1H-indazol-7-amine | C7 H7 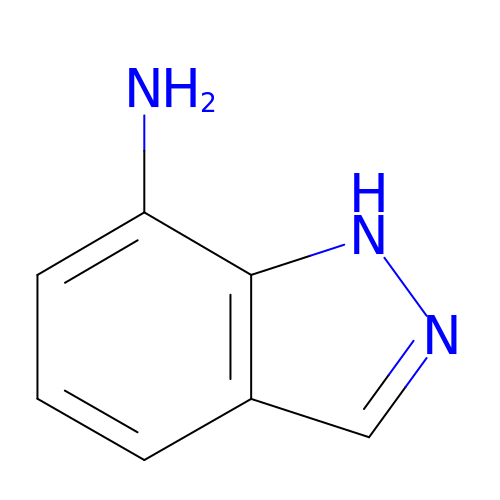N3 | OTFFCAGPSWJBDK-UHFFFAOYSA-N> RRTDEYILVRQTGQDKFAGTTKCNLDHLPTKAEFNASCRLYRDGVGNYYPPPLAFERIDLPEQLAAQLHNLEPREQSKQCF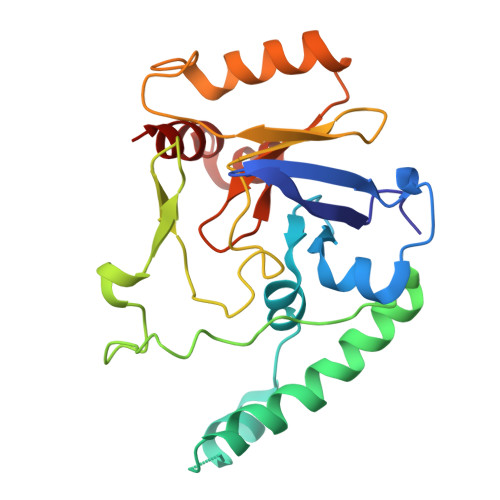QYKLEVWNRAHAEMGITGTDIFYQTDKNIKLDRNYKLRPEDRYIQTEKYGRREIQKRYEHQFQAGSLLPDILIKTPQNDIHFSYRFAGDAYANKRFEEFERAIKTKYGSDTEIKLKSKSGIMHDSKYLESWERGSADIRFAEFAG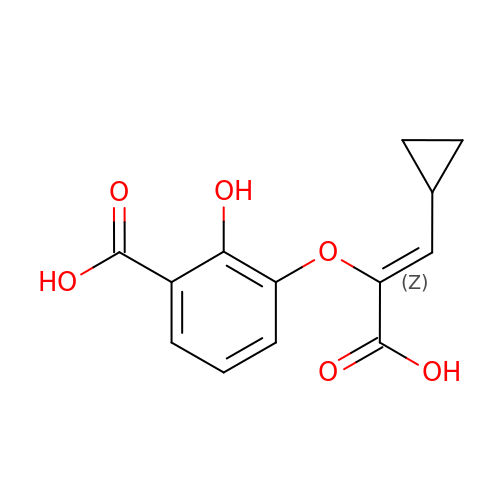3-{[(Z)-1-carboxy-2-cyclopropylethenyl]oxy}-2-hydroxybenzoic acid | C13 H12 O6 | RBBOJHGNWUPRCK-POHAHGRESA-N>MKPERKRVSKLMAYILRHSPEEFGLRPDVEGFVSLNELVNALKTVYPEVTEEFVREIVENDPAGRYEIRGDRIRARYGHSFPVSLDHEEDTESRFLYHGTPRRNLPSILKEGLKPMKRQYVHVSTDKIEALETGRRHGREV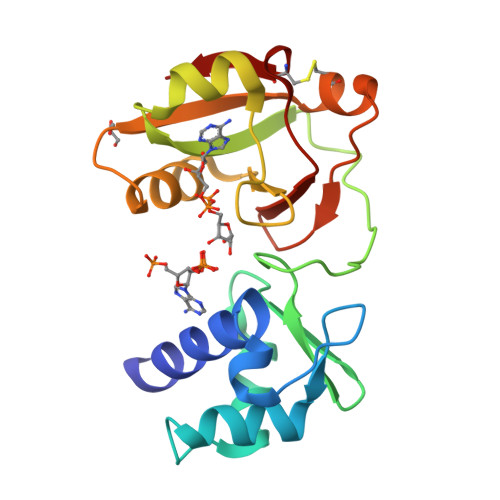VLLVIDAECLRKRGFKIYKAGKNVRIVERVPPDCITLAV[2x]DNA polymerase μ incorporates nucleotides in the non-homologous end-joining (NHEJ) pathway of double-strand break (DSB) repair. Error-prone synthesis by pol μ often introduces mismatches, as well as short deletions or insertions, at repaired sites. Pol μ is expected to frequently encounter oxidized nucleotides in its biological roles. We employed time-lapse X-ray crystallography to obtain snapshots of 8-oxodGTP insertion by pol μ on a model DSB substrate.

To explain these observations, we solved the structure of the pre-catalytic Ca2+:8-oxodGTP:Ct ground state ternary complex of the Lys438Asp variant. Surprisingly, 8-oxodGTP adopted the syn-conformation and formed Hoogsteen-like hydrogen bonds with Ct(anti). The primer terminus had rotated ~180° relative to wild type, while still stacking with the 8-oxodG(syn) base. O3′ of the rotated primer terminus was now stabilized by Ca2+ (instead of Na+) bound to the HhH motif through a water molecule. The loss of steric restraints due to removal of the primer terminus prompted Trp434 to rotate into the major groove. Apart from Lys438, active site interactions remained similar to wild type. Primer terminal instability appears to be hindered by Lys438, as the primer terminus is more readily displaced in the ground state 8-oxodGTP(syn):Ct(anti) ternary complex of the Lys438Asp variant. Lys438 provides steric constraints for the incoming nucleotide and primer terminus, as substitution of this residue with aspartate results in 8-oxodG(syn) and primer terminal displacement. Although 8-oxodGTP is accommodated in the active site in the syn-conformation opposite Ct in the absence of Lys438, efficient 8-oxodGTP:Ct insertion appears to require 8-oxodG to base-pair using the Watson–Crick edge. The role of Trp434 in active site stabilization is additionally revealed in the Lys438Asp mutant, where this residue contributed to modulation of catalysis by destabilizing the primer terminus.

> GSAAAPLSPAWMPAYACQRPTPLTHHNTGLSEALEILAEAAGFEGSEGRLLTFCRAASVLKALPSPVTTLSQLQGLPHFGEHSSRVVQELLEHGVCEEVERVRRSERYQTMKLFTQIFGVGVKTADRWYREGLRTLDDLREQPQKLTQQQKAGLQHHQDLSTPVLRSDVDALQQVVEEAVGQALPGATVTLTGGFRRGKLQGHDVDFLITHPKEGQEAGLLPRVMCRLQDQGLILYHQHQHSCCESPTRLAQQSHMDAFERSFCIFRLPQPGSWKAVRVDLVVAPVSQFPFALLGWTGSDLFQRELRRFSRKEKGLWLNSHGLFDPEQKTFFQAASEEDIFRHLGLEYLPPEQRNA> MAASCVLLHTGQKMPLIGLGTWKSEPGQVKAAIKYALTVGYRHIDCAAIYGNELEIGEALQETVGPGKAVPREELFVTSKLWNTKHHPEDVEPALRKTLADLQLEYLDLYLMHWPYAFERGDNPFPKNADGTIRYDATHYKDTWKALEALVAKGLVRALGLSNFSSRQIDDVLSVASVRPAVLQVECHPYLAQNELIAHCQARGLEVTAYSPLGSSDRAWRDPNEPVLLEEPVVQ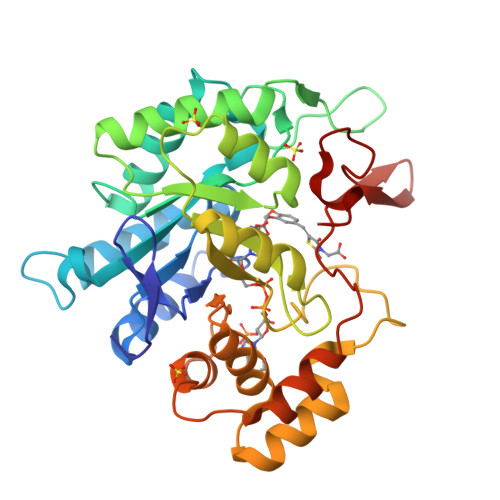ALAEKYNRSPAQILLRWQVQRKVICIPKSVTPSRILQNIQVFDFTFSPEEMKQLDALNKNLRFIVPMLTVDGKRVPRDAGHPLYPFNDPY>MQERRALRLGVNGLPNSLEPVNAISNVGPRIVNQIFDTLIARDFFAKGAPGNAIDLVPALAESWERIDEKSVRFKLRQKVMFHDGVELTADDVAYTFSSERLWGPEAIKKIPLGKSYSLDFDEPVVEDKYTVTLRTKTPSYLIETFVASWMSRIVPKEYYKKLGAVDFGNKPVGTGPYKFVEFVAGDRVVLEANDAYWGPKPTASKITYQIVAEPATRVAGLISGEYDIITTLTPDDIQLINSYPDLETRGTLIENFHMFTFNMNQEVFKDKKLRRALALAVNRPIMVEALWKKQASIPAGFNFPNYGETFDPKRKAMEYNVEEAKRLVKESGYDGTPITYHTMGNYYANAMPALMMMIEMWKQIGVNVVMKTYAPGSFPPDNQTWMRNWSNGQWMTDAYATIVPEFGPNGQVQKRWGWKAPAEFNELCQKVTVLPNGKERFDAYNRMRDIFEEEAPAVILYQPYDVYAARKDVHWKPVSFEMMEFRNNLSFGHHHHHH[4x]

To our knowledge, the best known system that exemplifies this paradigm is the antibiotic agrocin 84, which penetrates into the cytoplasm of the bacterial pathogen Agrobacterium tumefaciens strain C58 by hijacking the PBP called AccA and its cognate transporter. AccA also plays a key-role in the importation of the characteristic plant tumour-derived compounds such as the opines agrocinopines A and B discovered in 1981 in crown gall tumour tissue. The mature AccA structure is a monomer of 493 residues composed of two lobes, each formed by a central β-sheet flanked by α-helices. We identified the pyranose-2-phosphate-like moiety shared by these two ligands as the key recognition template for AccA.

The unliganded AccA structure solved at 1.7 Å resolution adopts an open conformation. Indeed, superposition with the liganded structures results in an average rmsd of 1.5 Å for all Cα atoms and structural comparisons show that upon ligand binding, a 12° rotation around an axis defined by the two hinge residues, Met292 and Tyr493, leads to a similar closed form of the protein. The biggest lobe (lobe 1) consists of residues 29–280 and 494–521 and the smallest (lobe 2) comprises the residues 285–489. The two lobes are connected by a very short hinge region of 8 residues defining two short segments.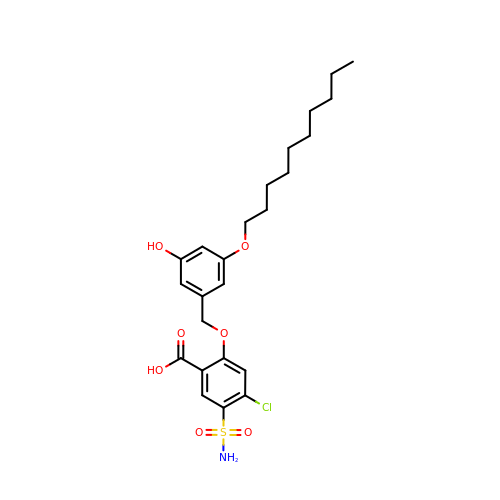4-chloro-2-{[3-(decyloxy)-5-hydroxybenzyl]oxy}-5-sulfamoylbenzoic acid | C24 H32 Cl N O7 S | ZGUBWBVFSMKCHM-UHFFFAOYSA-N>MKITVVDLGNINVKYVGENKGRFSSKITNDYQSYEEGFQRVEYNGIKTYIGVGELSREFNKADRDYMAQLLYSLAKANTADTKEINLTLLLPIIQMKNKTRLIETLKGENFKFKFNGIDREIKINDLMVLPEGYASYYSLDIENKKGDVCILDLGSRTINICVLENAKIVKTNTIKLGSFDFYSKIKSLENAKGEDYIEEDIQRLIDNGLIKVDSKQYIEFLSDILNAVKPYVNLKTYNTIFTGGTSLMLKEYIEKLPLNKFKVHPNALTSNVDGAMEASKKVWN[5x]

ParMs generally exist on low-copy number plasmids where they contribute to plasmid segregation and stable inheritance. Here we report the discovery and characterization of two chromosome-encoded ParMs (cParMs) from the genomes of Desulfitobacterium hafniense (Dh-cParM1) and Clostridium botulinum (Cb-cParM). Both cParMs form filaments, exhibit nucleotide hydrolysis, and possess characteristic ParM subunit structures.

We recorded CryoEM images of the Cb-cParM filaments after polymerization with ATP or GTP for 30 min. The averaged images of Cb-cParM, polymerized with ATP, revealed obvious wide and narrow regions along the filament, indicating a possible strand crossover. One map corresponds to the first condition (ATP, 30 min), at 3.9 Å resolution. The map from class 1 at 3.5 Å resolution (GTP, 30 min) was very similar to that from the first condition (ATP, 30 min). The two models from the two maps (ATP 30 min, and class 1 with GTP 30 min), were identical up to the reliable resolution of the data, despite the difference in the bound nucleotides. In both maps, density due to gamma phosphate or inorganic phosphate around the nucleotide was not observed, indicating that the bound nucleotides had been hydrolyzed to ADP and GDP, respectively, and the phosphate was released. The Cb-cParM filament reconstruction with ATP (30 min) was indistinguishable from that of class 1 with GTP (30 min). Phosphate release from Cb-cParM polymerized from ATP or GTP did not cause significant filament instability, as observed for other ParM systems, rather the filament underwent a significant structural change. The Cb-cParM cryoEM images showed obvious differences in the distribution of the nucleotide states between ATP and GTP at 30 min after initiation of polymerization. It implies either that phosphate release from the ADP-Pi state is faster than that from GDP-Pi state, or a faster rate of nucleotide hydrolysis, shortening time in the states of ADP-Pi and ATP in the nucleotide hydrolysis cycle.> SEEDRRLWMEAMDGREPVYNSNKDNQSEGTAQLDSIGFS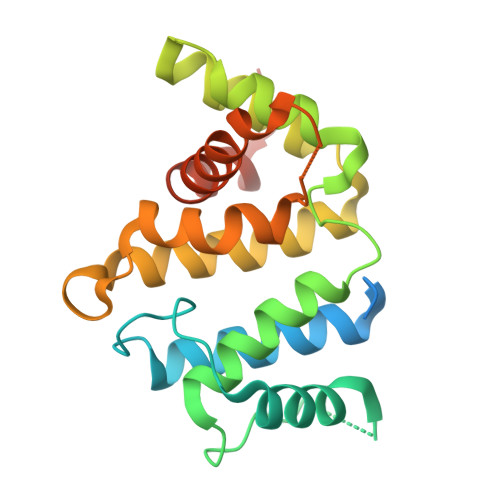IIKKCIHAVETRGINEQGLYRIVGVNSRVQKLLSILMDPKTATETETEICAEWEIKTITSALKTYLRMLPGPLMMYQFQRSFIKAAKLENQESRVSEIHSLVHRLPEKNRQMLHLLMNHLAKVADNHKQNLMTVANLGVVFGPTLLRPQEETVAAIMDIKFQNIVIEILIENHEKIFNTVPETPPSNSQLLL>[2x]MTTLHTIQLANPTECCTLATGPLSSDESEHYADLFKVLGDPVRLRILSQLAAGGCGPVSVNELTDLMGLSQPTISHHLKKMTEAGFLDRVPEG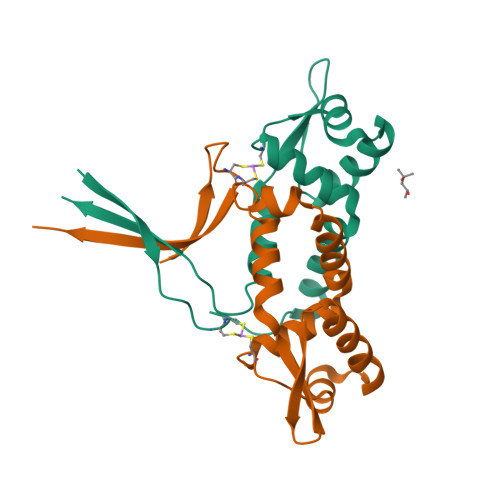RVVLHRVRPELFAELRTVLQIGSMELLEHHHHHH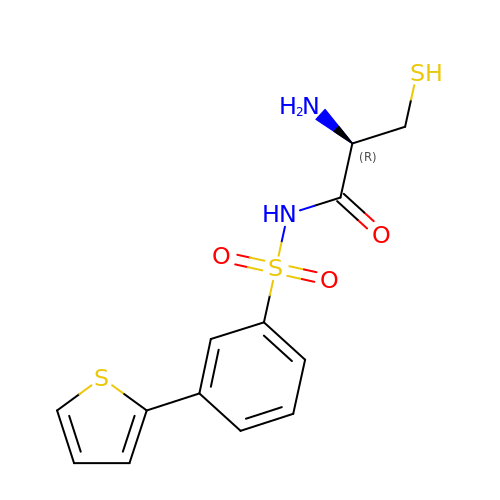N-[(3M)-3-(thiophen-2-yl)benzene-1-sulfonyl]-L-cysteinamide | C13 H14 N2 O3 S3 | SSWPXZNBBMHIKF-NSHDSACASA-N>MILNSFDLQGKVALITGCDTGLGQGMAIGLAQAGCDIVGVNIVEPKDTIEKVTALGRRFLSLTADMSNVSGHAELVEKAVAEFGHVDILVNNAGIIRREDAIEFSEKNWDDVMNLNIKSVFFMSQTVARQFIKQGKGGKIINIASMLSFQGGIRVPSYTASKSAVMGVTRLMANEWAKHGINVNAIAPGYMATNNTQQLRADEERSKEILDRIPAGRWGLPQDLMGPSVFLASSASDYIN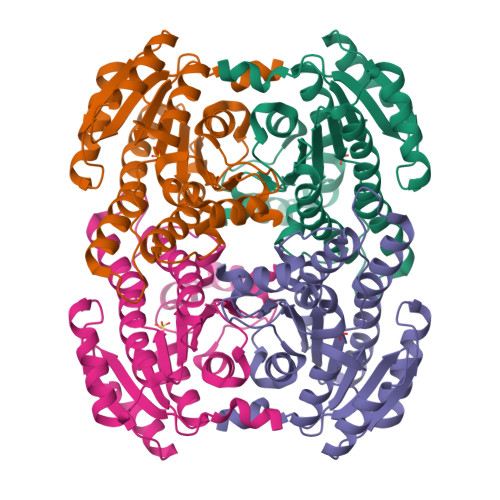GYTIAVDGGWLAR[4x]> MGSSHHHHHHSSGLVPRGSPWFGMDIGGTLVKLSYFEPIDITAEEEQEEVESLKSIRKYLTSNVAYGSTGIRDVHLELKDLTLFGRRGNLHFIRFPTQDLPTFIQMGRDKNFSTLQTVLC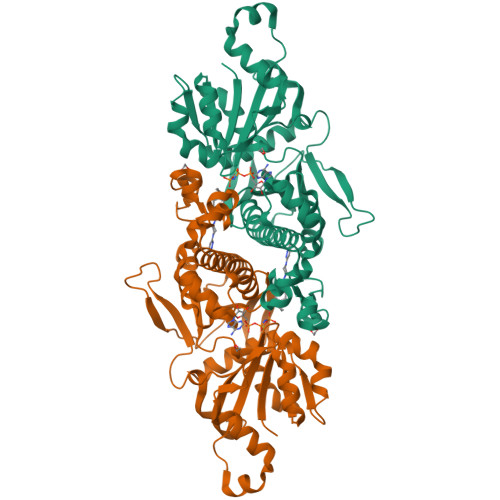ATGGGAYKFEKDFRTIGNLHLHKLDELDCLVKGLLYIDSVSFNGQAECYYFANASEPERCQKMPFNLDDPYPLLVVNIGSGVSILAVHSKDNYKRVTGTSLGGGTFLGLCSLLTGCESFEEALEMASKGDSTQADKLVRDIYGGDYERFGLPGWAVASSFGNMIYKEKRESVSKEDLARATLVTITNNIGSVARMCAVNEKINRVVFVGNFLRVNTLSMKLLAYALDYWSKGQLKALFLEHEGYFGAVGALLGLPNFSDD[(1R)-1-amino-2-(benzylamino)ethyl]phosphonic acid | C9 H15 N2 O3 P | 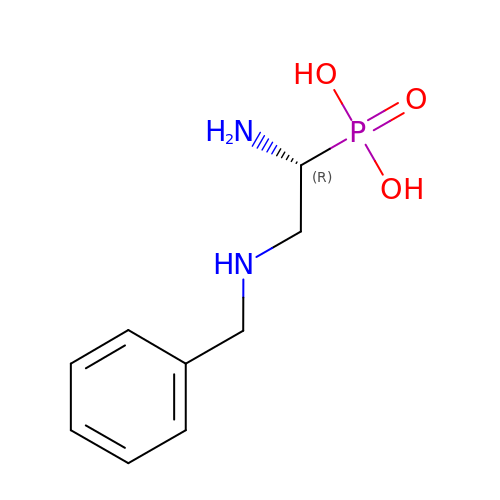TYSJLDXCWVWYDI-SECBINFHSA-N> MVDQATLDKLEAGFKKLQEASDCKSLLKKHLTKDVFDSIKNKKTGMGATLLDVIQSGVENLDSGVGIYAPDAESYRTFGPLFDPIIDDYHGGFKLTDKHPPKEWGDINTLVDLDPAGQFIISTRVRCGRSLQGYPFNPCLTAEQYKEMEEKVSSTLSSMEDELKGTYYPLTGMSKATQQQLIDDHFLFKEGDRFLQTANACRYWPTGRGIFHND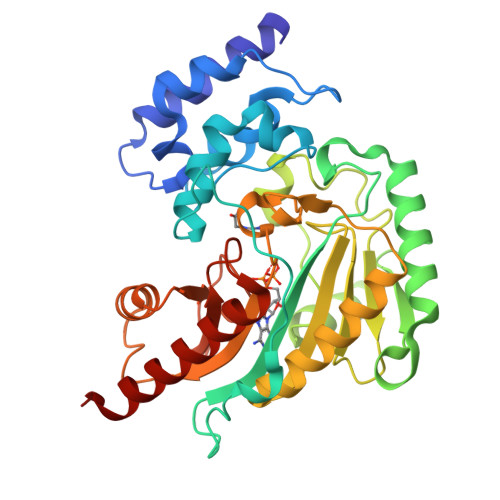AKTFLVWVNEEDHLRIISMQKGGDLKTVYKRLVTAVDNIESKLPFSHDDRFGFLTFCPTNLGTTMRASVHIQLPKLAKDRKVLEDIASKFNLQVRGTRGEHTESEGGVYDISNKRRLGLTEYQAVREMQDGILEMIKMEKAAA> MKILTQDEIEAHRSHTLKGGIEGALAGFAISAIIFKVLPRRYPKFKPSTLTWSIKTALWITPP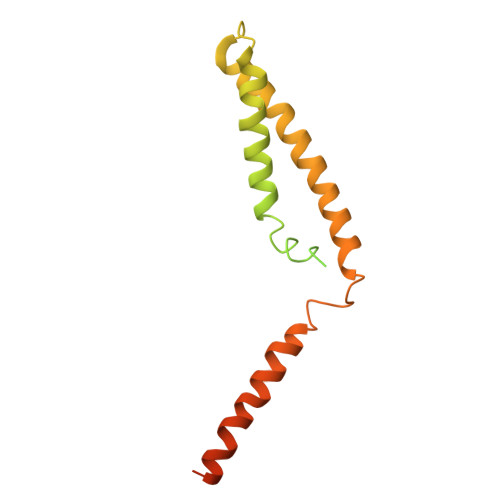TVLTAICAEEASNNFDATMYGSGSSSEDALDEHRRWKSLSTKDKFVEGLSNNKYKIITGAWAASLYGSWVIVNKDPIMTKAQKIVQARMYAQFITVGLLLASVGLSMYENKLHPNKQKVNEMRRWENALRVAEEEERLEKEGRRTGYVSNEERINSKIFKS> QFAKPEDAVKYRQSAATLMASHFGRMTPVVKGQAPYDAAQIKANVEVLKTLSALPWAAFGPGTEGGDARPEIWSDAASFKQKQQAFQDNIVKLSAAADAGDLDKLRAAFGDVGASCKACHDAYRK

Cytochromes c′ occur in methanotrophic, denitrifying and photosynthetic bacteria and have proposed roles in protection against nitrosative stress, NO trafficking during denitrification or pathogen defence. All cytochromes c′ have a 4 α-helix bundle structure containing a heme centre with a solvent exposed proximal His ligand and a buried hydrophobic distal pocket with a non-coordinated residue (Leu or Phe, rarely Met or Tyr) in a position to exert steric influence on the binding of diatomic gases. Unusually, cytochromes c′ are able to utilize both heme faces (distal and proximal) as a means of discriminating NO from other diatomic gases. In order to understand the factors controlling distal versus proximal NO coordination, we have examined NO binding to AXCP variants in which the occluding distal residue Leu16 is replaced with residues that are smaller (Ala, Val), of comparable size (Ile) or larger (Phe).

All of the tertiary structures are similar to wt AXCP and only salient points concerning the heme region are discussed here. Ferrous structures show the different residues at position 16 to lie over the heme in a similar manner to that of Leu16 in wt AXCP (Fig. S4†) with the exception of L16A where the side chain is essentially truncated.> GSHIEGYECQPIFLNVLEAIEPGVVCAGHDNNQPDSFAALLSSLNELGERQLVHVVKWAKALPGFRNLHVDDQMAVIQYSWMGLMVFAMGWRSFTNVNSRMLYFAPDLVFNEYRMHKSRMYSQCVRMRHLSQEFGWLQ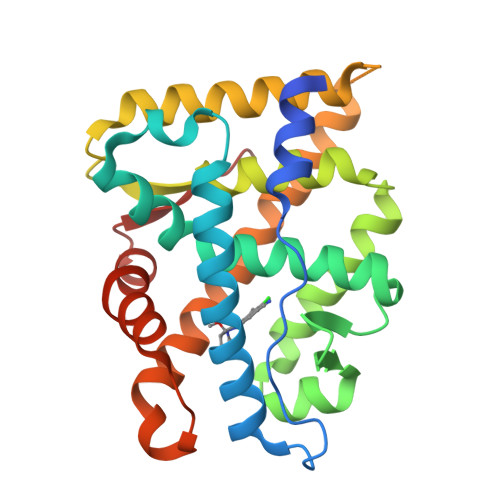ITPQEFLCMKALLLFSIIPVDGLKNQKFFDELRMNYIKELDRIIACKRKNPTSCSRRFYQLTKLLDSVQPIARELHQFTFDLLIKSHMVSVDFPEMMAEIISVQVPKILSGKVKPIYFHTQ> MESVERKSESSYLGMRNMQPEQRLSLDPPRLRSTPQDELHDLLCVGFGPASLAIAIALHDALDPRLNKSASNIHAQPKICFLERQKQFAWHSGMLVPGSKMQISFIKDLATLRDPRSSFTFLNYLHQKGRLIHFTNLSTFLPARLEFEDYMRWCAQQFSDVVAYGEEVVEVIPGKSDPSSSVVDFFTVRSRNVETGEISARRTRKVVIAIGGTAKMPSGLPQDPRIIHSSKYCTTLPALLKDKSKPYNIAVLGSGQSAAEIFHDLQKRYPNSRTTLIMADSAMRPSDDSPFVNEIFNPERVDKFYSQSAAERQRSLLADKATNYSVVRLELIEEIYNDMYLQRVKNPDETQWQHRILPERKITRVEHHGPQSRMRIHLKSSKPESEGAANDVKETLEVDALMVATGYNRNAHERLLSKVQHLR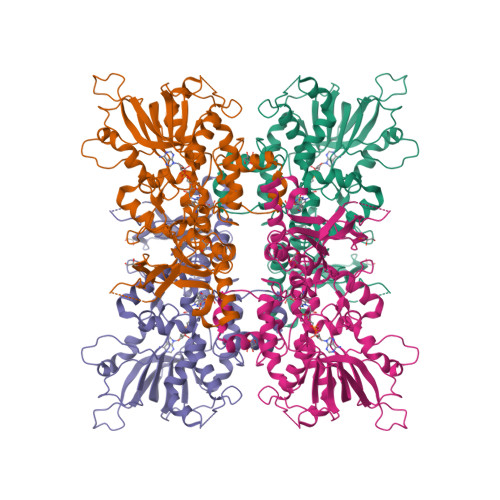PTGQDQWKPHRDYRVEMDPSKVSSEAGIWLQGCNERTHGLSDSLLSVLAVRGGEMVQSIFGEQLERAAVQGHQLRAML>[5x]NAMIIRPEQHWFLRLFDWHGSVLSKIIFRLLLNVLMSIIAIISYQWYEQLGIHLTVAPFSLLGIAIAIFLGFRNSASYSRFVEARNLWGTVLIAERTLVRQLRNILPAEHDAHRRIVSY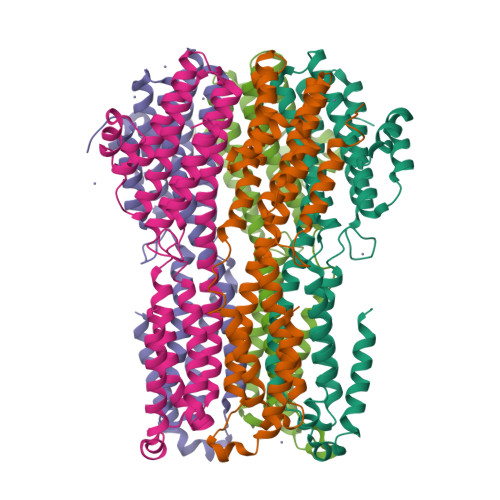LVAFSWSLKHQLRKTDPTADLRRLLPEERVTEILASSMPTNRILLLAGNEIGQLREAGKLSDATYGLMDNKLDELAHVLGGCERLATTPVPFAYTLILQRTVYLFCTLLPFALVGDLHYMTPFVSVFISYTFLSWDSLAEELEDPFGTAANDLPLNAMCNTIERNLLDMTGQHPLPE>[2x]MSKPQPIAAANWKCNGSQQSLSELIDLFNSTSINHDVQCVV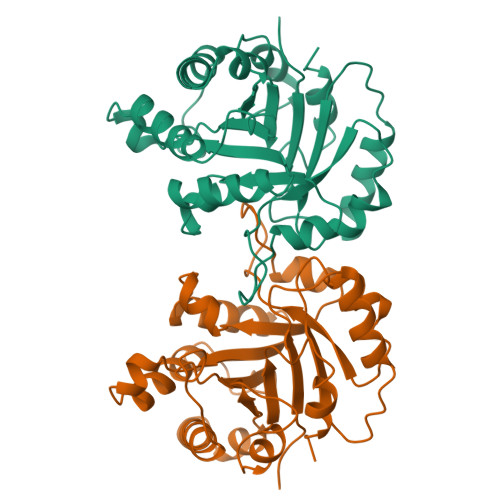ASTFVHLAMTKERLSHPKFVIAAQNAIAKSGAFTGEVSLPILKDFGVNWIVLGHSERRAYYGETNEIVADKVAAAVASGFMVIACIGETLQERESGRTAVVVLTQIAAIAKKLKKADWAKVVIAYEPVWAIGTGKVATPQQAQEAHALIRSWVSSKIGADVRGELRILYGGSVNGKNARTLYQQRDVNGFLVGGASLKPEFVDIIKATQ>[2x]GSDPTQFEERH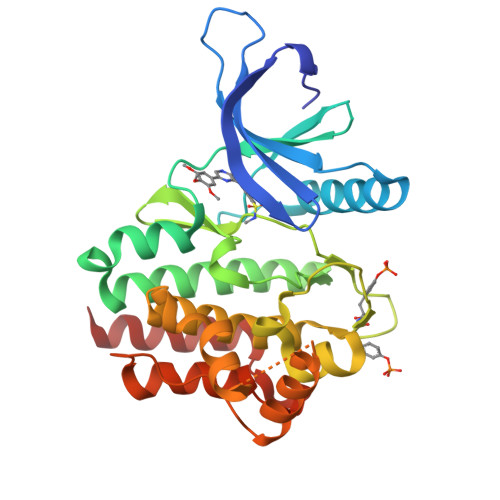LKFLQQLGKGNFGSVEMCRYDPLQDNTGEVVAVKKLQHSTEEHLRDFEREIEILKSLQHDNIVKYKGVCYSAGRRNLKLIMEYLPYGSLRDYLQKHKERIDHIKLLQYTSQICKGMEYLGTKRYIHRDLATRNILVENENRVKIGDFGLTKVLPQDKEYYKVKEPGESPIFWYAPESLTESKFSVASDVWSFGVVLYELFTYIEKSKSPPAEFMRMIGNDKQGQMIVFHLIELLKNNGRLPRPDGCPDEIYMIMTECWNNNVNQRPSFRDLALRVDQIRDNMAG(1S,2S,3R,6R)-4-(hydroxymethyl)-6-(octylamino)cyclohex-4-ene-1,2,3-triol | C15 H29 N O4 | 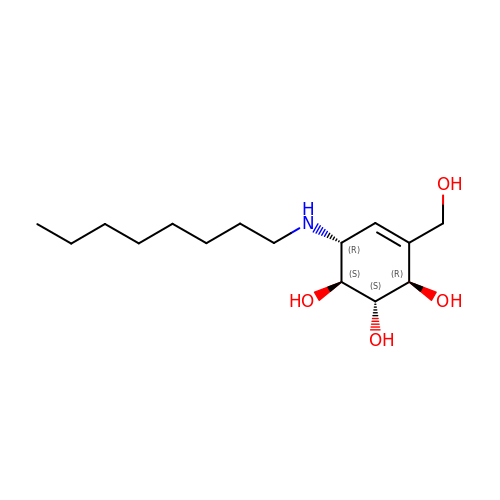UPZUHYMBTUUPML-KBXIAJHMSA-N>GMDKYREIHNKLKEFSPGTLTAVECIDYLDRLYAVRHDIVDQMIKHDWSDNKDSEEAIGKVLLFAGVPSNIITALEKKIIPNHPTGKSLKAFFKMTPDNYKISGTTIEFVEVTVTADVDKGIREKKLKYEAGLTYIEQELHKFFLKGEIPQPYKITFNVVAVRTDGSNITTQWPSRRNDG[2x]

Segmented negative strand RNA viruses of the arena-, bunya- and orthomyxovirus families uniquely carry out viral mRNA transcription by the cap-snatching mechanism. This involves cleavage of host mRNAs close to their capped 5′ end by an endonuclease (EN) domain located in the N-terminal region of the viral polymerase. The sNSV cap-snatching ENs belong to the PD-D/ExK superfamily of cation dependent nucleases. We find two different kinds of endonucleases, one with the characteristic catalytic histidine (His+) as in orthomyxovirus and bunyavirus, which have efficient endonuclease activity in isolation, and a second, without the histidine (His-) and conserved among arenaviruses which shows very poor activity in vitro.

To demonstrate the presence of a cap-snatching endonuclease domain in hantavirus L proteins we determine the crystal structure of the isolated Hantaan virus EN in complex with Mn2+ ions and characterize its endonuclease activity. We could express and purify protein constructs comprising residues 1–179 and 1–182 that crystallized with 2 mM MnCl2 as thick plates diffracting to 1.7 Å resolution. The structure was solved by SAD experiment. Each protein binds two Mn2+ ions in the active site in a similar fashion to that observed for LACV and influenza. A third Mn2+ stabilises the interface between crystallographic symmetry related neighbour proteins. Overall, Hantaan EN conserves the two lobe shape of LACV but with the active site, which lies between the two lobes, being more accessible. The active site of Hantaan EN structure is configured very similarly to that of LACV and IAV ENs with two divalent cations bound in a canonical way. Mn1 is octahedrally coordinated by the side chains of amino acid residues H36, D97 (from the conserved PD motif) and E110, and the main chain carboxyl oxygen of V111. Mn2 is coordinated by D97 and E54 coming from the conserved flexible loop preceding helix αc. The Hantaan EN efficiency for single stranded RNA appears similar to IAV and LACV but it is able to cleave structured RNA more efficiently than either IAV or LACV, probably due to the higher accessibility to the active site.> SMHSDLTFCEIILMEMESHDAAWPFLEPVNPRLVSGYRRIIK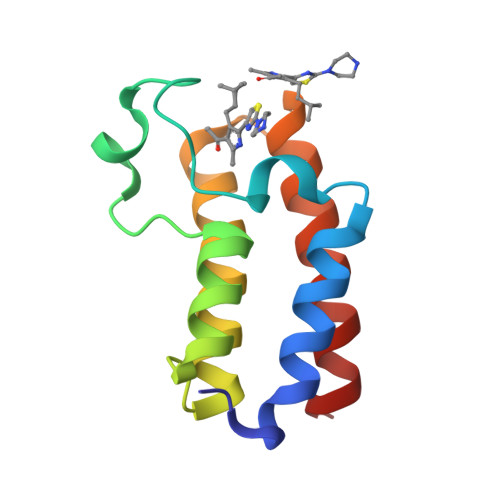NPMDFSTMRHRLSRGGYTSSEEFAADALLVFDNCQTFNEDDSEVGKAGHIMRRFFESRWEEFYQ>TPDCVTGKVEYTKYNDDDTFTVKVGDKELATNRANLQSLLLSAQITGMTVTIKTNACHNGGGFSEVIFR[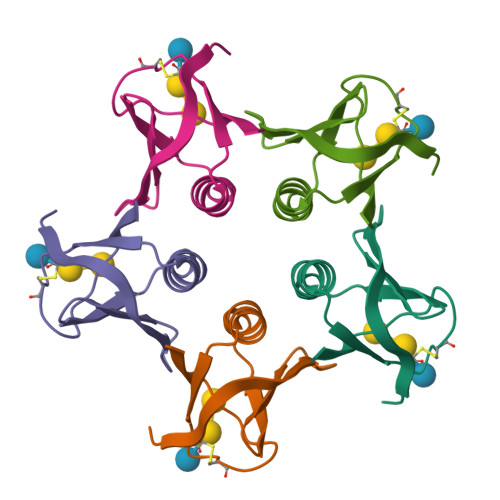5x]> ESLQRKRLCKARLYDVTRHHVKHKRLKPLIEHIDEYCNEKDENKGDVLFFLLRSHLYDTGNRSMAEQIDTLWHGESLSCMTPEECLGMRLDMLMTKNQYSKEYNILKERGFSTLCPPKQLDAIEKTLMPGTARYSIEGMDYSEHYFHSPVKMTGDLEVHSGETLEPDSVTMDFHEYVPDFPCPNTKGVRFPYAHAVAKTLEELEDEIVNGLKKLGRDPNDPTLVIHTICKDGADGMGDVSVHKEKSDHLLPDKALRFSFCVLRCSVMHKDTEVTIYEDPNPNSVRSNRPVLECIGDENDDGTVAVCVGPIECQRLLMKDKIMRVHMSDGTQRAHYLTFFNSMVDEKWDRAHGGLAGAGSKYLCTLCEAVRDEALEKAGSYKITRTLKKIEVTASKMKYESQEKDTFGVKGYPLLTTEPWERGIDATHTDINMGNYFKSLIVREMAQVHSWAKTANVKKQIVDAESKLDKHLKESLGLNPTLMMAGNYARELFKAEHADKLVALVDKPDRKSALVEVLAKFRQLRKVYRANWPLNDMSDEVRQYKAKAVEMANDLKTHFPYAPCTNYLHKVIEHVQELIEHPSGVGS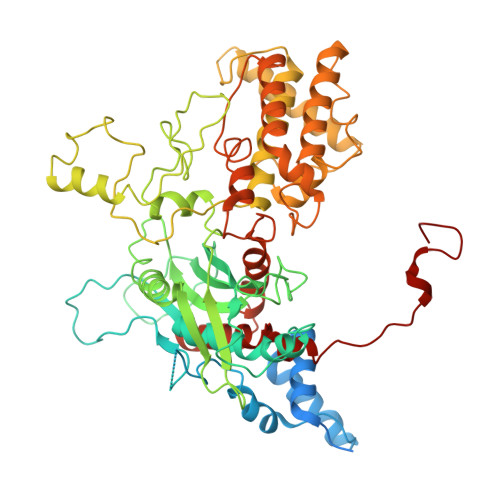VGALSSEGNEAGNKLFRQLRLGHARKGNTYNGLRDVLCTHWLYTSKTLRDKAAXXXXXXXXXXXXXXXXXXX> MRSSKIRCPGAIRVGTLVTAFGCLPHVAFAAAREAPPVTPEVLVRLADIGTMSASETTPLLSLSPDGRYVAFQVRQADPVTNLNVFRMVVKATDGATDAIDVDVGGEYLFWTIPSWGYARNAPSGANLTIQPRWSPSGTHLAYLRQDQGRVRVWRASVKGEGASPVIEDAYDIEDVQWLDDNTLIYSGRPGFVEAEAEIEREGRRGWVYDERFHPLTGARPRVLEPISIVYQVLDLKTGTRRAATPTEVARLREKPDPLRAMVGRTTFSVSRTDPQNINAPTTLVARRGEGEPVRCDEEACQNITRMWGDETANVLYFLRREGWASNEMALYRMPADALKPVRIWHATGLLQGCERQAKRLICAQESALQPRRLVTLNLTSGQMSPLYDPNPDLSRYRLPKVERLTLRNRNGIEVFSDLVLPPDYQLGTRLPLVIVQYSSRGFLRGGTGDENPILPLATAGFAVLSFHSPRSEASYQRFTSPI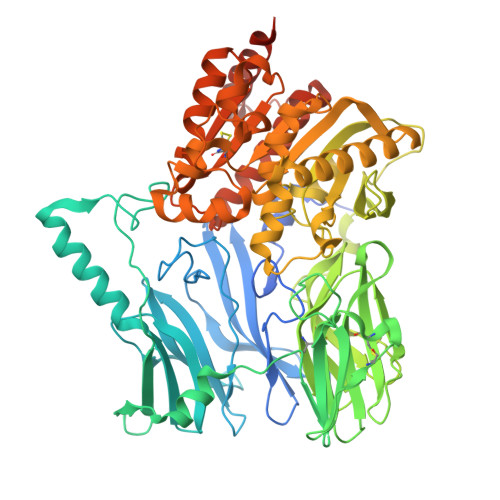AQSKAEYSNWRNRWNILHTLEDLIDDLDRRGVIDPARVGLTGLADGATTVHFGLINSHRFAAAVTSSCCTDSFTASVMNGPRISGALKAYGIETDQADDGPFWAATSFVVNASRLDTPLLIQSADEEYLGALPGFTALQQARKPVELIIYPNEHHVKWQPAHRLAVYNRTIDWFRFWLMDQSDPAPDKAAQYDRWRALRALRQKSPSPTPAPGSRSHHHHHH>QAVTAFLGERVTLTSYWRRVSLGPEIEVSWFKLGPGEEQVLIGRMHHDVIFIEWPFRGFFDIHRSANTFFLVVTAANISHDGNYLCRMKLGETEVTKQEHLSVVKPLTLSVHSERSQFPDFSVLTVTCTVNAFPHPHVQWLMPEGVEPAPTAANGGVMKEKDGSLSVAVDLSLPKPWHLPVTCVGKNDKEEAHGVYVSGYLSQ[3x];>DPSEYCSHMIGSGHLQSLQRLIDSQMETSCQITFEFVDQEQLKDPVCYLKKAFLLVQDIMEDT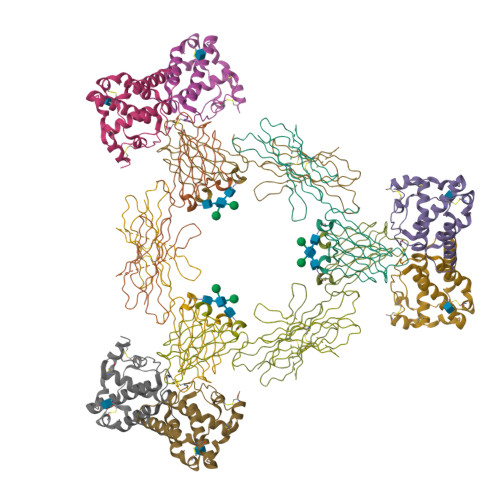MRFRDNTPNAIAIVQLQELSLRLKSCFTKDYEEHDKACVRTFYETPLQLLEKVKNVFNETKNLLDKDWNIFSKNCNNSFAECSS[3x]> MNTNNIKKYAPQARNQFRDAVIQKLTTLGISADKKGNLQIADAELVGETMRYGQFDYPKSTLTRRDRLVKRAREQGFDVLVEHCAYTWFNRLCAIRYMEIHGYLDHGFHMLSHPDNPTGFEVLDHVPEVAEALLPEKKAQLVEMKLSGNQDEAIYRELLLAQCHALHRAMPFLFEAVDDEAELLLPDNLTRTDSILRGLVDGIPEEDWQEVEVIGWLYQFYISEKKDAVIGKVVKSEDIPAATQLFTPNWIVQYLVQNSVGRQWLQTYPDSPLKGKMDYYIEPAEQTPEVQAQLAAITPASIEPESIKVLDPACGSGHILIEVYNVLKNIYEERGYRARDIPQLILENNIFGLDIDDRAAQLSGFALLMMARQDDRRIFTRDVRLNIVSLQESLHLDIAKLWQQLNFHQQNQTGSMGDMFAENTALAHTDSAEYQLLMRTLKRFVNAKTLGSLIQVPQEEEAELKAFLEALYRMEQ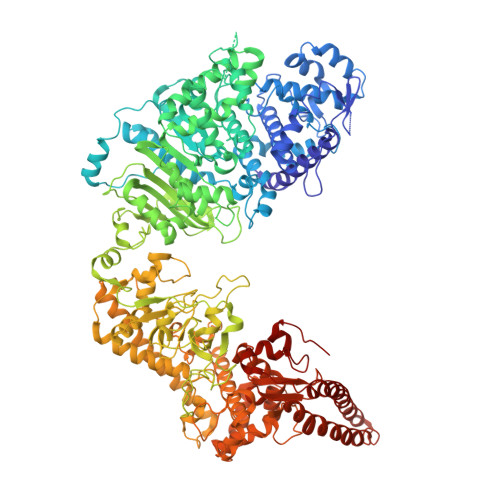EGDFQQKAAAKAFIPYIQQAWILAQRYDAVVANPPYMGGKGMNSELKEFAKNNFPDSKADLFAMFMQNAFSLLKENGFNAQVNMQSWMFLSSYEALRNWLLDNKTFITMAHLGARAFGQISGEVVQTTAWVIKNQHSERYQPVFFRLIDGREEVKKSDLLLRKNIFDKFTQHDFKNIPGMPIAYWIDLPSLLSFRHHKKLGEKIALKAGMSTGDNIKFQRYWYEVSIKKTLITNKESNTKIDIHNIKWFPCSSGGEYRKWYGNNEIVVNWENNGYEIRNFKFENGKTRSAVRNDEYYFREGITWSKISQGNFCVRYRPKGFVFDDTGRCGFSNNKNELLYAAGLMCTPVVNHYLSILAPTLSFTSGELASVPYPEIEDEIIELVTNAIEIAKNDWDSQEQSWDYVCSPLLEHNSTQLLRNIYKQKINTNIKLVETLLLIENTINNIFIDKLQLDKTIIKAVLQSEITLLCNPNYRYKNIQDHTDLTNKYYTDITIDILSYIIGCMMGRYSLDREGLVYAHEGNKGFAELVAEDAYKTFPADNDGILPLMDDEWFDDDVTSRVKEFVRTVWGEEHLQENLEFIAESLCLYAIKPKKGESALDTIRRYLSTQFWKDHMKMYKKRPIYWLFSSGKEKAFECLVYLHRYNDATLARMRTEYVVPLLARYQANIDRLNEQVDGASGGEATRLKRERDSLSKKFNELRSFDDRLRHYADMRISIDLDDGVKVNYGKFGDLLADVKAITGNAPEII1-[2-(3-ACETYL-2-HYDROXY-6-METHOXY-PHENYL)-CYCLOPROPYL]-3-(5-CYANO-PYRIDIN-2-YL)-THIOUREA 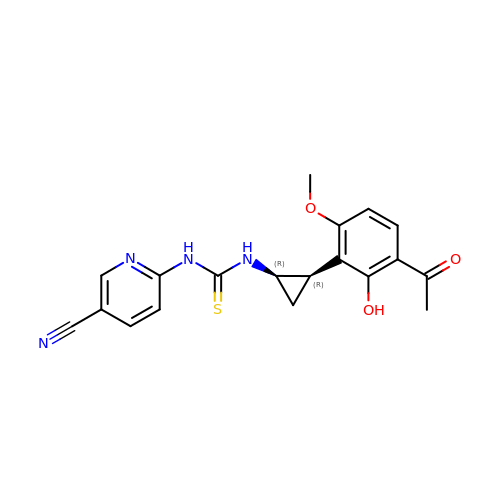| C19 H18 N4 O3 S | FSRLCMRWYUJTNT-UONOGXRCSA-N> MELKNLTVAIATFFASTNALALSEPSQQVTEIYQHHAHQNGNDRALPDYAPTKLLPQQPKPTLRTLSTRSAEQAANVCDVEAFTSNSSNDVLNAIKTQGASCVNALFSAESRIQEAAFESGHMYNIAKHTTDLAKAYAGGGSDELEALFLYLRAGYYAEFYNSKVSFLSWVTPAVKEAVDAFVNNANFYENSDPHGKVLSEVIITMDSAGLQHAYLPQVTQWLTRWDSQYAQNWYMRNAVNGVFTILFGGQWNEQFVQTIGNQTELAKALGDFALRSSAIGASDEFMAANAGRELGRLTKYSGSASSTVKSKLTEIFAQYEMYGRGDAIWLGAADTVS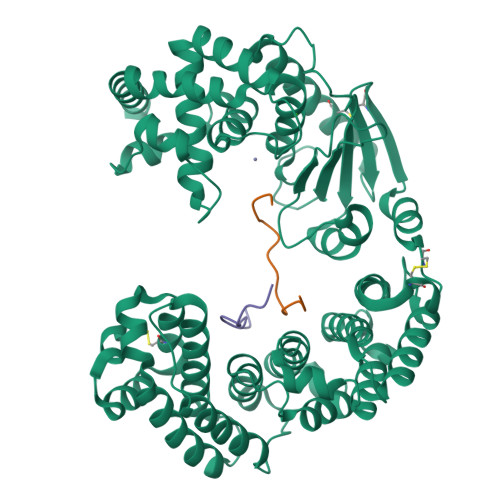YYADCSDYGICNFESQLKGLVLSQSYTCSPTIRILSQNMTQDQHVAACSKMGYEEGYFHTSLETGRQPVADDYNTQLQVNIFDSSDDYGKYAGPIFNISTNNGGMYLEGDPATPGNIPNFVAYEAPYANPDHFVWNLEHEYVHYLDGRFDLYGGFGHPTERIVWWSEGIAEYVSKENDNQAAIDTIKDGSTFTLSEIFETSYDGFDVDRIYRWGYLAVRFMFERHKDDVNQMLIETRQGNWANYKATINQWAILYQSEFEQWQQALVLEHHHHHH;> EPSQQVTEIYQHHA;> DYAPTKLLPQQP>EKIPIIVGDYGPMWVYPTSTFDCVVADPRKGSKMYGLKSYIEYQLTPTNTNRSVNHRYKHFDWLYERLLVKFGSAIPIPSLPDKQVTGRFEEEFIKMRMERLQAWMTRMCRHPVISESEVFQQFLNFRDEKEWKTGKRKAERDELAGVMIFSTMEPEAPDLDLVEIEQKCEAVGKFTKAMDDGVKELLTVGQEHWKRCTGPLPKEYQKIGKALQSLATVFSSSGYQGETDLNDAITEAGKTYEEIASLVAEQPKKDLHFLMECNHEYKGFLGCFPDIIGTHKGAIEKVKESDKLVATSKITLQDKQNMVKRVSIMSYALQAEMNHFHSNRIYDYNSVIRLYLEQQVQFYETIAEKLRQALSRFPVM[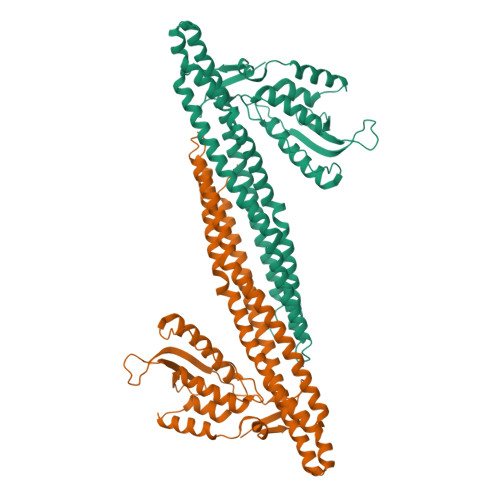3x]>PGSKPFSVPVLTVEEMTNSRFPIPLEKLFTGPSSAFVVQPQNGRCTTDGVLLGTTQLSPVNICTFRGDVTHITGSRNYTMNLASQNWNNYDPTEEIPAPLGAPDFVGKIQGMLTQTTRADGSTRGHKATVYTGSADFAPKLGRVQFETDTDHDFEANQNTKFTPVGVIQDGSTTHRNEPQQWV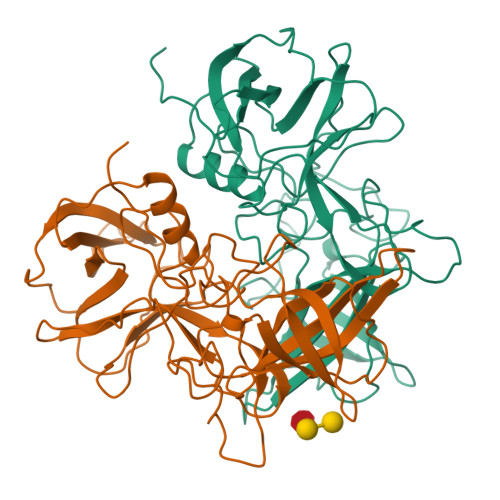LPSYSGRNTHNVHLAPAVAPTFPGEQLLFFRSTMPGCSGYPNMDLDCLLPQEWVQYFYQEAAPAQSDVALLRFVNPDTGRVLFECKLHKSGYVTVAHTGQHDLVIPPNGYFRFDSWVNQFYTLAPM[2x]> IGTGFPFDPHYVEVLGERMHYVDVGPRDGTPVLFLHGNPTSSYVWRNIIPHVAPTHRCIAPDLIGMGKSDKPDLGYFFDDHVRFMDAFIEALGLEEVVLVIHDWGSALGFHWAKRNPERVKGIAFMEFIRPIPTWDEWPEFARETFQAFRTTDVGRKLIIDQNVFIEGTLPCGVVRPLTEVEMDHYREPFLNPVDREPLWRFPNELPIAGEPANIVALVEEYMDWLHQSPVPKLLFWGTPGVLIPPAEAARLAKSLPNCKAVDIGPGLNLLQEDNPDLIGSEIARWLSTLEISG

Therefore, we aimed to develop a genetically encodable click reaction (GEN-Click) system that can selectively target the CuAAC reaction catalyst proximal to the protein of interest and that can be genetically expressed in live cells. To selectively tag the Cu(I)-binding catalyst on the protein of interest, we employed two different methods for protein modification using genetic tag proteins. One method used the HaloTag,14−16 which can be selectively conjugated with chloroalkane-conjugated ligands. Therefore, we developed the “GEN-Click” system, which can target the copper(I)-catalyzed azide/alkyne cycloaddition reaction catalysts proximal to the protein of interest and can be genetically expressed in a live cell.

To test our GEN-Click approach using HaloTag, we synthesized a chloroalkane-based HaloTag ligand (HTL) conjugated to a BTTA moiety connected by poly(ethylene glycol) (PEG) linkers of various lengths (BTTA-PEGn-HTL). Our BTTA-PEG-HTL ligands exhibited favorable HaloTag binding properties, as confirmed in a competitive binding assay. However, the BTTA-HTL ligand did not show high CuAAC catalytic activity for azidocoumarin and propargyl alcohol as a substrate when bound to HaloTag, despite showing good catalytic activity in the free form. Our crystal data suggest that the specific surface residues of HaloTag strongly inhibit copper complexation of BTTA via π–π or hydrogen-bonding events at the surface. As expected, HaloTag-TM expressing cells showed no desthiobiotin-alkyne labeling with BTTA-HTL.>MASSTFYIPFVNEMGEGSLEKAIKDLNGSGFKNALIVSDAFMNKSGVVKQVADLLKAQGINSAVYDGVMPNPTVTAVLEGLKILKDNNSDFVISLGGGSPHDCAKAIALVATNGGEVKDYEGIDKSKKPALPLMSINTTAGTASEMTRFCIITDEVRHVKMAIVDRHVTPMVSVNDPLLMVGMPKGLTAATGMDALTHAFEAYSSTAATPITDACALKAASMIAKNLKTACDNGKDMPAREAMAYAQFLAGMAFNNASLGYVHAMAHQLGGYYNLPHGVCNAVLLPHVLAYNASVVAGRLKDVGVAMGLDI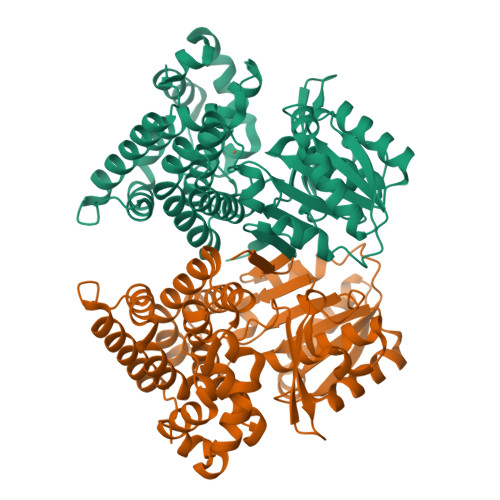ANLGDKEGAEATIQAVRDLAASIGIPANLTELGAKKEDVPLLADHALKDACALTNPRQGDQKEVEELFLSAF[4x]1-[(1S)-1-(2-fluorophenyl)ethyl]piperazine | C12 H17 F N2 | 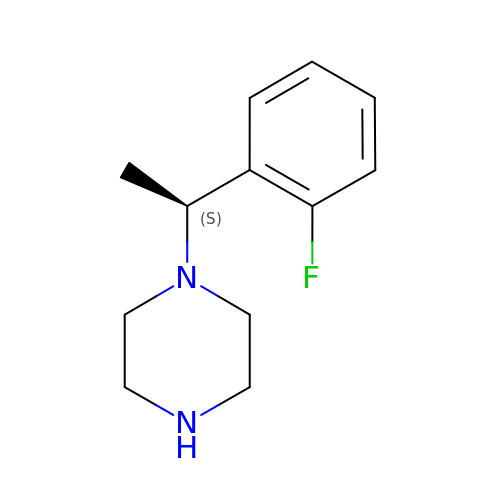UIJNEACQJVSKLI-JTQLQIEISA-N> METRSDVFEFEFSETPLLPCYNIQVSVAQGPRNWLLLSDVLKKLKMSSRIFRCNFPNVEIVTIAEAE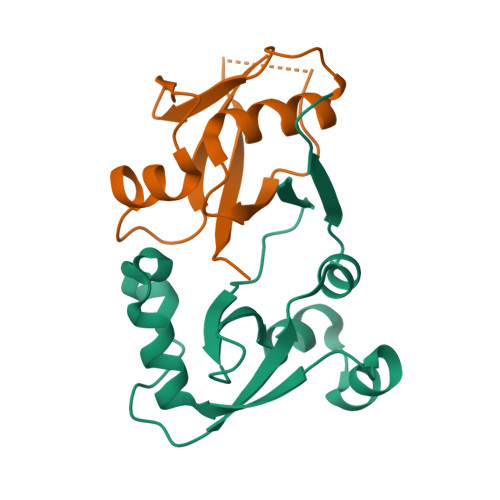FYRQVSASLLFSCSKDLEAFNPESKELLDLVEFTNEIQTLLGSSVEWLHPSD;> QGTREQLNLCLERLSSGKDKNKSVLQNKYVRCSVRAEVRHLRRVLCHRLMLNPQHVQLLFDNEVLPDHMTMKQIWLSRWFGKPSPLLLQYSVK> AGAGAAGAAAGGGA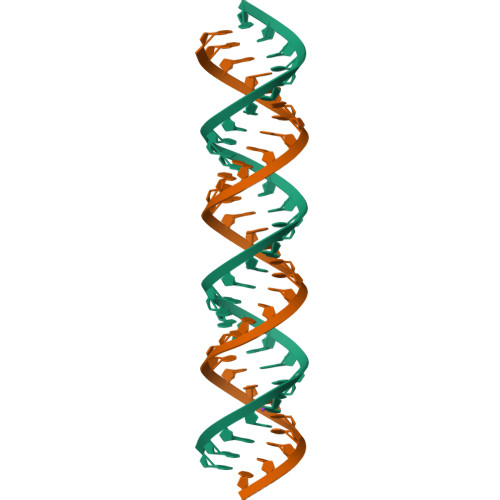AAUUUUUUUUUUUUUUUU>TEGWFMPFDNWLYQLQNADPVEISSSGFEIAVIDYSKDGSESGEYSPEEIKIMVDAGVVPVAYVNIGQAEDYRFYWKES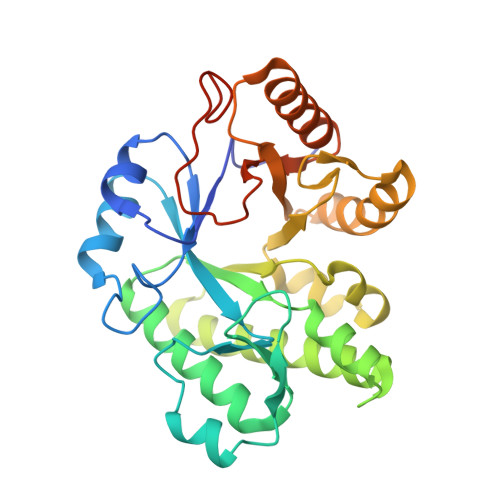WYTNTPEWLGEEDPAWPGNYFVKYWYNEWKEIVFSYLDRVIDQGFKGIYLDRIDSFEYWAQEGVISRRSAARKMINFVLEIAEYVRERKPDMLIIPQNGENILDFDDGQLASTVSGWAVENLFYLKTIPLEENETKSRLEYLIRLNRKGKFILSVDYVDDGSDSFENISRILDYYEKAKRNGCIPYAARSDLELDEMNVIEGIQPPEALKDYESRTYR[6x]> MEANGLGPQGFPELKNDTFLRAAWGEETDYTPVWCMR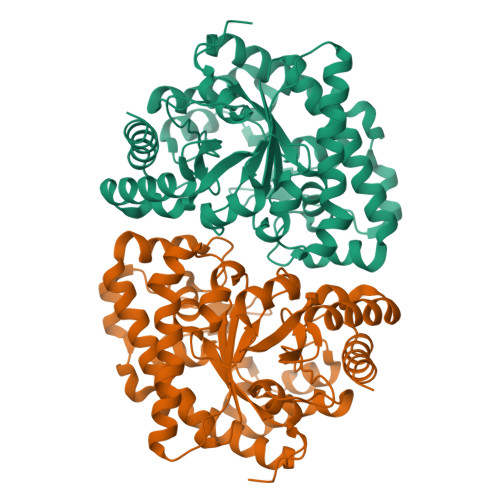QAGRYLPEFRETRAAQDFFSTCRSPEACCELTLQPLRRFPLDAAIIFSDILVVPQALGMEVTMVPGKGPSFPEPLREEQDLERLRDPEVVASELGYVFQAITLTRQRLAGRVPLIGFAGAPWTLMTYMVEGGGSSTMAQAKRWLYQRPQASHQLLRILTDALVPYLVGQVVAGAQALQLFESHAGHLGPQLFNKFALPYIRDVAKQVKARLREAGLAPVPMIIFAKDGHFALEELAQAGYEVVGLDWTVAPKKARECVGKTVTLQGNLDPCALYASEEEIRQLVKQMLDDFGPHRYIANLGHGLYPDMDPEHVGAFVDAVHKHSRLLRQN> VGDDSGGFSTTVSTEQNVPDPQVGITTMRDLKGKANRGKMDVSGVQAPVGAITTIEDPVLAKKVPETFPELKPGESRHTSDHMSIYKFMGRSHFLCTFTFNSNNKEYTFPITLSSTSNPPHGLPSTLRWFFNLFQLYRGPLDLTIIITGATDVDGMAWFTPVGLAVDTPWVEKESALQIDYKTALGAVRFNTRRTGNIQIRLPWYSYLYAVSGALDGLGDKTDSTFGLVSIQIANYNHSDEYLSFSCYLSVTEQSEFYFPRAPLNSNAMLSTESMMSR;> DIEEEQMIQSVDRTAVTGASYFTSVDQSSVHTAEVGSHQIEPLKTSVDKPGSKKTQGEKFFLIHSARWLTTHALFHEVAKLDVVKLLYNEQFAVQGLLRYHTYARFGIEIQVQINPTPFQQGGLICAMVPGDQSYGSIASLTVYPHGLLNCNINNVVRIKVPFIYTRGAYH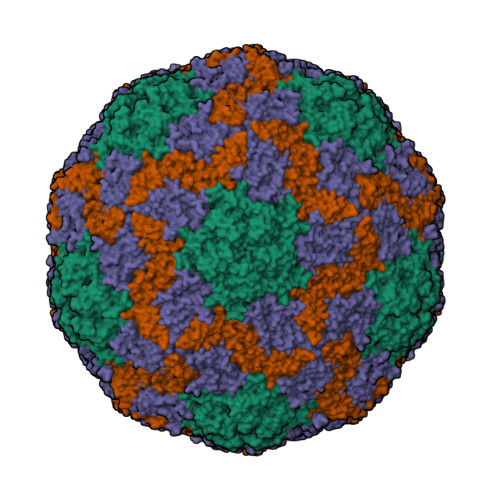FKDPQYPVWELTIRVWSELNIGTGTSAYTSLNVLARFTDLELHGLTPLSTQ;> MMRNETRVSTTENVVNLSNYEDARAKMSFALDQEDWKSDPSQGGGIKITHFTTWTSIPTLAAQFPFNASDSVGQQIKVIPVDPYFFQMTNTNPDQKCITALASICQMFCFWRGDLVFDFQVFPTKYHSGRLLFCFVPGNELIDVTGITLKQATTAPCAVMDIAGVQSTLRFRVPWISDTPYRVNRYTKEAHQKGEYTAIGKLIVYCYNRLTSPSNVAHHVRVNVYLSAINLECFAPLYHAMDVTTQ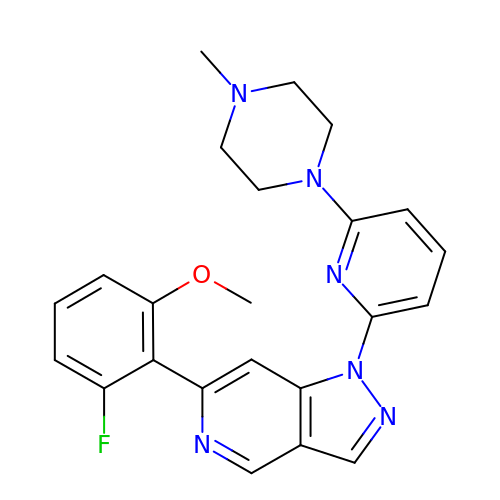6-(2-fluoro-6-methoxyphenyl)-1-[6-(4-methylpiperazin-1-yl)pyridin-2-yl]-1H-pyrazolo[4,3-c]pyridine | C23 H23 F N6 O | KAOYHQWWTGUIBS-UHFFFAOYSA-N> RVQSGKINCGDDAGWAKVPSNDPGRDNTRELAKNITFASPYCRPPVVLLSITQLDVEQSQNLRVIARLYSVSPTGFKASCYTWHNTKVYSMSI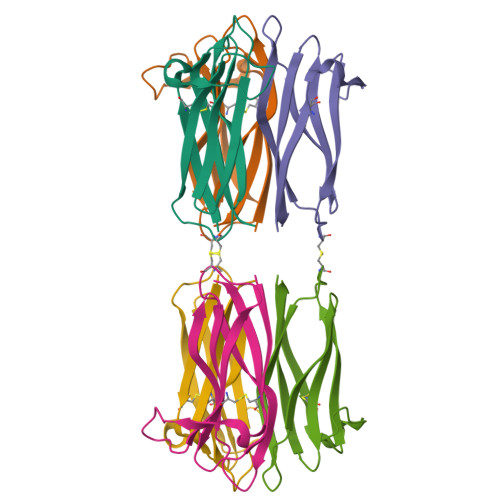SWISIENY14-methylhexadec-9-enoic acid | C17 H32 O2 | 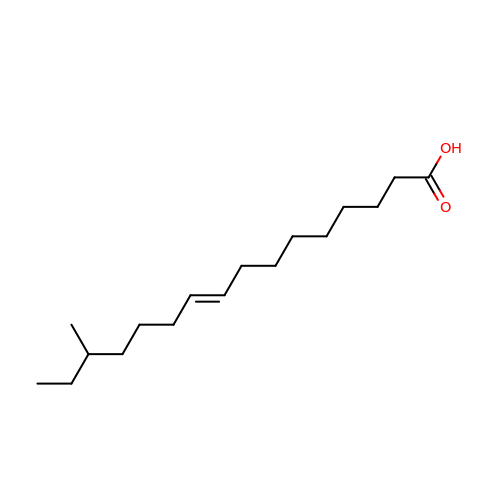JSOOUDKFWVPPEF-UHFFFAOYSA-N> XSGGLQVKNFDFTVGKFLTVGGFINNSPQRFSV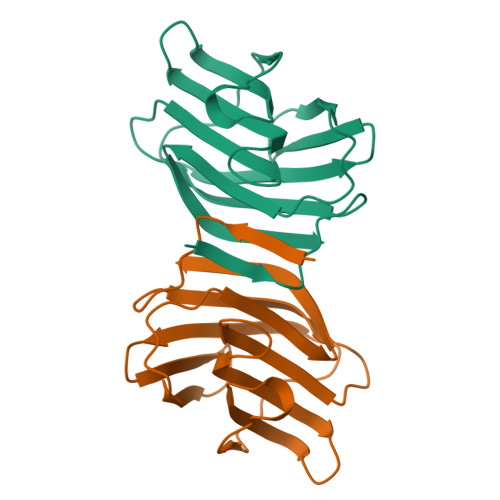NVGESMNSLSLHLDHRFNYGADQNTIVMNSTLKGDNGWETEQRSTNFTLSAGQYFEITLSYDINKFYIDILDGPNLEFPNRYSKEFLPFLSLAGDARLTLVKLE>ARERGHNFERMKIKTPTKCGHCTSILIGLDRQGLFCQSCQYACHVSCAERVSQSCPVPEEERRPLGIDPTRGVGTAYEGLVKTPRAGGVRKGWQTAYVVVCDFKLYLYDCTVDRQNKMQDVKNEIRLVLDMRDPDFTVCGVSEADVIHAQKGDIPKIFRVTTTQILNSSSEYSSSSKFYTLFMAETEEEKRKWVVALSELKTLLRRSKLADRKAFLVKEVFDVTTLPSIRVAQCCAIIDRSKIVIGFSDHGLYCIEISRQLLIPVGGEKENKQRCVETVEYDEAEQLLMMIVGPAKDRHVRIVPSAALDGRDLKWIKVNDTKGCHLLAVGTNNPGGRAGFFAVAFKKSVTIFQIDRSEKRHKKWKDLAMPGTPQSIAIFNGRLYVGFSHSFRSWSLVGVDSSPVGSGDASGAVLQHISLVNMEDTSLQFLNQQTSYEAKLIVNVPGSPDEYLLVFNMIGLYVNEMGRRSRLPEVMFPTQAKYFAYHEPYLCVFSENEVDIFNVTLAEWVQTINLRSAKPLSGDGILSTCLCNDSPIFVLLQNVLQDQDSIEVPVNLASGSTDGRKVTRRKFTF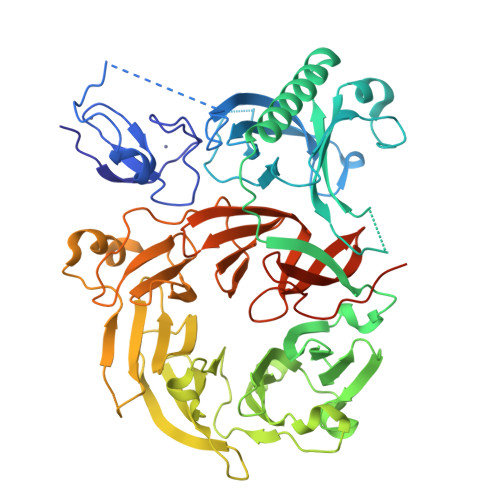RTIGKDDRS[5x]> MERMLPLLALGLLAAGFCPAVLCHPNSPLDEENLTQENQDRGTHVDLGLASANVDFAFSLYKQLVLKAPDKNVIFSPLSISTALAFLSLGAHNTTLTEILKGLKFNLTETSEAEIHQSFQHLLRTLNQSSDELQLSMGNAMFVKEQLSLLDRFTEDAKRLYGSEAFATDFQDSAAAKKLINDYVKNGTRGKITDLIKDLDSQTMMVLVNYIFFKAKWEMPFDPQDTHQSRFYLSKKKWVMVPMMSLHHLTIPYFRDEE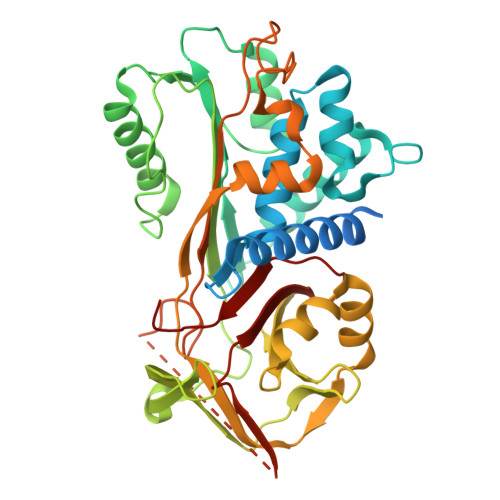LSCTVVELKYTGNASALFILPDQDKMEEVEAMLLPETLKRWRDSLEFREIGELYLPKFSISRDYNLNDILLQLGIEEAFTSKADLSGITGARNLAVSQVVHKAVLDVFEEGTEASAATAVKITLLSALVETRTIVRFNRPFLMIIVPTDTQNIFFMSKVTNPKQA Peptidyl-prolyl isomerases (PPIases) catalyze cis/trans isomerization of peptidyl-prolyl bonds, which is often rate-limiting for protein folding. SlyD is a two-domain enzyme containing both a PPIase FK506-binding protein (FKBP) domain and an insert-in-flap (IF) chaperone domain. In order to improve our understanding of the mechanism of SlyD and of FKBPs in general, we set out to analyze the kinetics, energetics, and structural basis for substrate binding and inhibition of SlyD from Thermus thermophilus (TtSlyD) using 15-residue-long unmodified peptides, which we reasoned would be better mimics of natural unfolded protein substrates than the traditionally used 4-nitroanilide tetrapeptides. In total, we obtained five structures of TtSlyDFL and three of TtSlyDΔIF at a maximum resolution of up to 1.4 Å.

Finally, we also analyzed binding of the S2, S3, and mutated variants of the S2 peptide to a chimeric TtSlyD construct, in which the IF domain is replaced by the flap loop from human FKBP12 (henceforth abbreviated TtSlyDΔIF). In addition, we carried out co-crystallization with the FKBP inhibitor FK506. FK506 binds in a similar way to all three copies of TtSlyD in the asymmetric unit of TtSlyDFL:FK506 and in both copies in TtSlyDΔIF:FK506, but exhibits some structural variation in parts of the molecule that are more distal to the binding pocket. The binding mode is similar to that observed in the FK506–FKBP12 complex. Specifically, the pipecolinyl ring, which mimics a proline side chain, is inserted into the center of the hydrophobic pocket, and four hydrogen bonds are formed: two to the backbone of N35 and I37 (V55 and I56 in FKBP12), and one each to the side chains of D23 and Y63 (D37 and Y82 in FKBP12). Most noteworthy are three potential interactions between the C9 carbonyl oxygen of FK506 and CH groups of Y13, L15, and F128, which are reminiscent of three putative CH–O interactions observed between FK506 and FKBP12 residues Y26, F36, and F99. As discussed further below, this variability is intimately connected with interactions between the side chain of Y63 and the peptides bound to the FKBP domain. The FKBP12 flap loop inserted into TtSlyDΔIF in place of the IF domain adopts essentially the same conformation as in full-length FKBP12 in the case of TtSlyDΔIF:FK506, while it is partially disordered in TtSlyDΔIF:S2-W23A and TtSlyDΔIF:S3. It furthermore shows that the pipecolinyl ring partially overlaps with the side chain of cis-P29S2 in both peptide binding modes, but is in a roughly orthogonal orientation relative to these, which enables it to reach considerably deeper into the pocket. In addition, we also found that FK506 forms two hydrogen bonds that mimic the β-strand type hydrogen bonds formed by the peptides.

>MKVGQDKVVTIRYTLQVEGEVLDQGELSYLHGHRNLIPGLEEALEGREEGEAFQAHVPAEKAYGATGHPGIIPPHATLDFQVEVVKVREATPEELLHGHAHPSGHHHHHH[2x]>[6x]SMPPVFDENEDVNFDHFEILRAIGKGSFG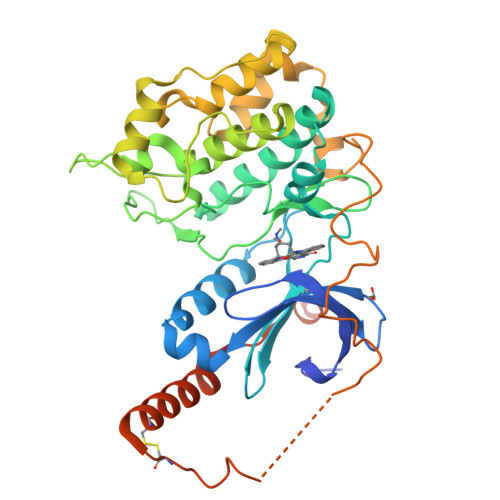KVCIVQKNDTKKMYAMKYMNKQKCVERNEVRNVFKELQIMQGLEHPFLVNLWYSFQDEEDMFMVVDLLLGGDLRYHLQQNVHFKEETVKLFICELVMALDYLQNQRIIHRDMKPDNILLDEHGHVHITDFNIAAMLPRETQITTMAGTKPYMAPEMFSSRKGAGYSFAVDWWSLGVTAYELLRGRRPYHIRSSTSSKEIVHTFETTVVTYPSAWSQEMVSLLKKLLEPNPDQRFSQLSDVQNFPYMNDINWDAVFQKRLIPGFIPNKGRLNCDPTFELEEMILESKPLHKKKKRLAKKEKDMRKCDSSQTCLLQEHLDSVQKEFIIFNREKVNRDFNKRQPNLALEQTKDPQGED>[2x]MS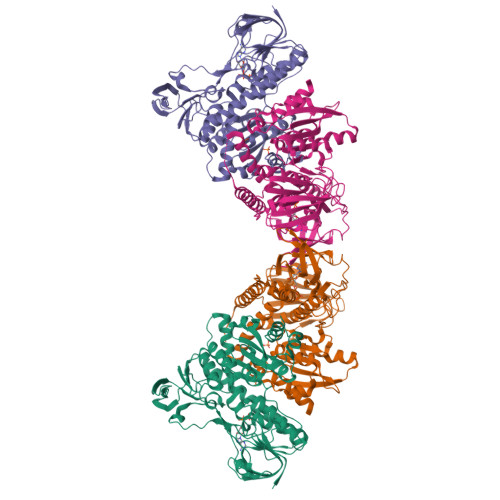LKYDVVVIGAGGAGYHGAFRLAKAKYNVLMADPKGELGGNCLYSGCVPSKTVREVIQTAWRLTNIANVKIPLDFSTVQDRKDYVQELRFKQHKRNMSQYETLTFYKGYVKIKDPTHVIVKTDEGKEIEAETRYMIIASGAETAKLRLPGVEYCLTSDDIFGYKTSFRKLPQDMVIIGAGYIGLEIASIFRLMGVQTHIIEMLDRALITLEDQDIVNTLLSILKLNIKFNSPVTEVKKIKDDEYEVIYSTKDGSKKSIFTNSVVLAAGRRPVIPEGAREIGLSISKTGIVVDETMKTNIPNVFATGDANGLAPYYHAAVRMSIAAANNIMANGMPVDYVDVKSIPVTIYTIPSLSYVGILPSKARKMGIEIVEAEYNMEEDVSAQIYGQKEGVLKLIFERGSMRLIGAWMIGVHSQYLINELGLAVAYGLNAKQLASFAEQHPSTNEIISYTARKVIEGHHHHHH> MGTFTLHQGQTNLIKSFFRNYYLNAELELPKDMELREFALQPFGSDTYVRHLSFSSSEELRDYLVNRNLPLHLFYSSARYQLPSARNMEEKAWMGSDLLFDIDADHLCKLRSIRFCPVCGNAVVSEKCERDNVETLEYVEMTSECIKRGLEQTRNLVEILEDDFGLKPKVYFSGNRGFHVQVDCYGNCALLDSDERKEIAEYVMGIGVPGYPGGSENAPGWVGRKNRGINGVTIDEQVTIDVKRLIRIPNSLHGKSGLIVKRV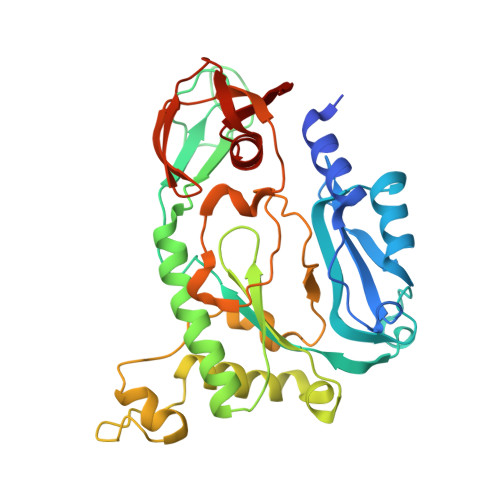PNLDDFEFNETLSPFTGYTIFLPYITIETEVLGSIIKLNRGIPIKIKSSIGIYLHLRNLGEVKAYVR> TGTSTVGVGRGVLGDQKNINTTYSTYYYLQDNTRGDGIFTYDAKYRTTLPGSLWADADNQFFASYDAPAVDAHYYAGVTYDYYKNVHNRLSYDGNNAAIRSSVHYSQGYNNAFWNGSEMVYGDGDGQTFIPLSGGIDVVAHELTHAVTDYTAGLIY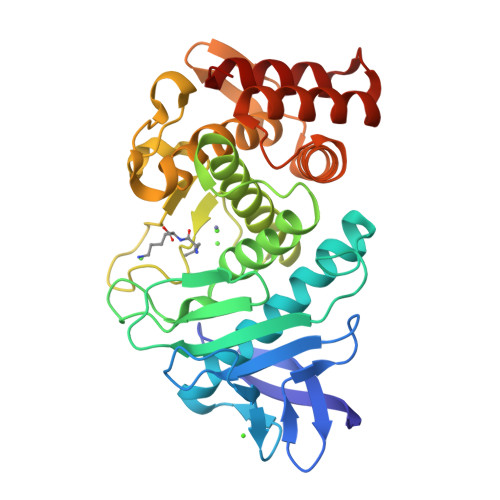QNESGAINEAISDIFGTLVEFYANKNPDWEIGEDVYTPGISGDSLRSMSDPAKYGDPDHYSKRYTGTQDNGGVHINSGIINKAAYLISQGGTHYGVSVVGIGRDKLGKIFYRALTQYLTPTSNFSQLRAAAVQSATDLYGSTSQEVASVKQAFDAVGVK>AQYEDGKQYTTLEKPVAGAPQVLAFFSFFCPHCYQFEEVLHISDNVKKKLPEGVKMTAYHVNFMGGDLGKDLTQAWAVAMALGVEDKVTVPLFEGVQKTQTIRSASDIRDVFINAGIKGEEYDAAWNSFVVKSLVAQQEKAAADVQLRGVPAMFVNGKYQLNPQGMDTSNMDVFVQQYADTVKYLSEKK[2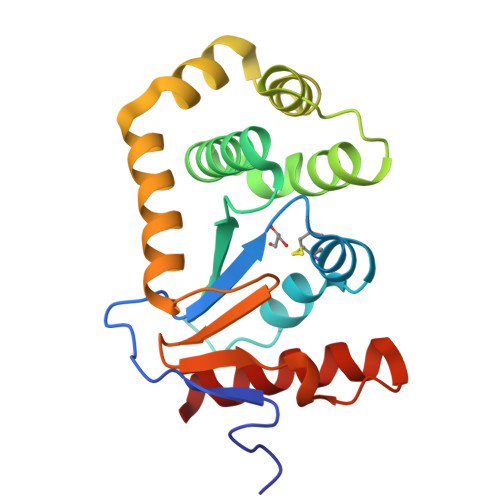x]Mature CVB1 virions, like other enteroviruses, have 4 structural proteins termed viral protein 1–4 (VP1–4). They form an icosahedrally-symmetric capsid of about 30 nm in diameter with VP1 around the 5-fold, VP2 on the sides of the 2-fold and alternating VP2 and VP3 around 3-fold symmetry axes. At the base of VP1, there is a hydrophobic pocket which normally contains a lipid factor. Similar to empty particles, recombinantly produced Virus-Like Particles (VLPs) closely mimic the structure of infectious virions but lack genetic material.

Through cryoEM and single-particle image processing, two distinct particle populations were separated. These particle populations were termed compact and expanded, structurally corresponding to mature native CVB1 virions and CVB1 A-particles respectively. Particle distribution is 48–52% in favor of the expanded particles. There is no density corresponding to VP4 of VP0 in the expanded CVB1-VLPTween80 structure and no significant unmodeled density which would suggest a flexible region. Residues on the VP3 loop are rotated away from the pore on the side of the 2-fold, potentially not blocking the VP1 N-terminus exit from the capsid. Unmodelled density shown at threshold of 1.5 σ above mean on the sides of the 2-fold outside the capsid could be flexible VP1 N-terminus. At the current resolution, an ion coordinated between three D203 at the 3-fold can be observed in both expanded and compact forms. In the expanded CVB1-VLPsTween80, a forked density is present above cysteins which could be additional ion densities and in the compact CVB1-VLPTween80 two conformations of VP3 R232 are resolved. Here we observed two structural differences of CVB1-VLPsTween80 compared to native CVB1 which are the presence of a VP3 loop in the pore of the expanded CVB1-VLPsTween80 and an additional density in the interprotomer pocket of compact CVB1-VLPTween80.

> SRSESSIENFLCRAACVYYATYTNNSEKGYAEWVINTRQVAQLRRKLELFTYLRFDLELTFVITSAQQPSTATSVDAPVQTHQIMYVPPGGPVPTKVTDYAWQTSTNPSVFWTEGNAPPRMSIPFISIGNAYSCFYDGWTQFSRNGVYGINTLNNMGTLYMRHVNEAGQGPIKSTVRIYFKPKHVKAWVPRPPRLCQYEKQKNVNFTPTGVTTTRVGITT;> RVRSITLGNSTITTQECANVVVGYGVWPEYLKDNEATAEDQPTQPDVATCRFYTLESVQWMKNSAGWWWKLPDALSQMGLFGQNMQYHYLGRTGYTIHVQCNASKFHQGCLLVVCVPEAEMGCSNLNNTPEFAELSGGDTARMFTDTQIGETNSKKVQTAVWNAGMGVGVGNLTIYPHQWINLRTNNSATIVMPYINSVPMDNMFRHNNLTLMIIPFVPLNYSEGSSPYVPITVTIAPMCAEYNGLRLA;> GLPVMTTPGSTQFLTSDDFQSPSAMPQFDVTPEMQIPGRVNNLMEIAEVDSVVPVNNTEANVNSLKAYQIPVQSNSDNGKQVFGFPLQPGANGVLNRTLLGEILNYYTHWSGSIKLTFMFCGSAMATGKFLLAYSPPGAGVPKNRKDAMLGTHVIWDVGLQSSCVLCVPWISQTHYRYVVEDEYTAAGYITCWYQTNIVVPADVQSSCDILCFVSACNDFSVRMLKDTPFIR> MDKFRVQGPTKLQGEVTISGAKNAALPILFAALLAEEPVEIQNVPKLKDVDTSMKLLSQLGAKVERNGSVHIDARDVNVFCAPYDLVKTMRASIWALGPLVARFGQGQVSLPGGCTIGARPVDLHISGLEQLGATIKLEEGYVKASVDGRLKGAHIVMDKVSVGATVTIMCAATLAEGTTIIENAAREPEIVDTANFLITLGAKISGQGTDRIVIEGVERLGGGVYRVLPDRIETGTFLVAAAISRGKIICRNAQPDTLDAVLAKLRDAGADIEVGEDWISLDMHGKRPKAVNVRTAPHPAFPTDMQ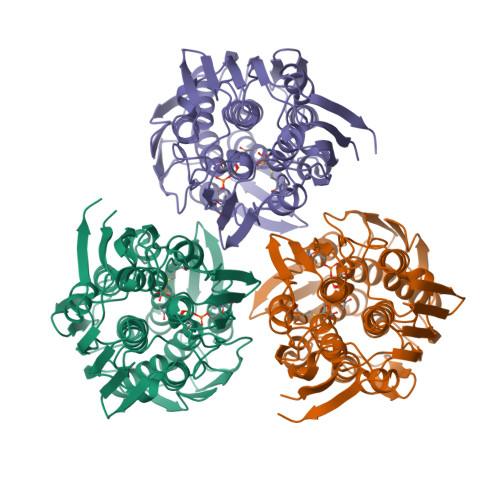AQFTLLNLVAEGTGFITETVFENRFMHVPELSRMGAHAEIESNTVICHGVEKLSGAQVMATDLRASASLVLAGCIAEGTTVVDRIYHIDRGYERIEDKLRALGANIERVKGE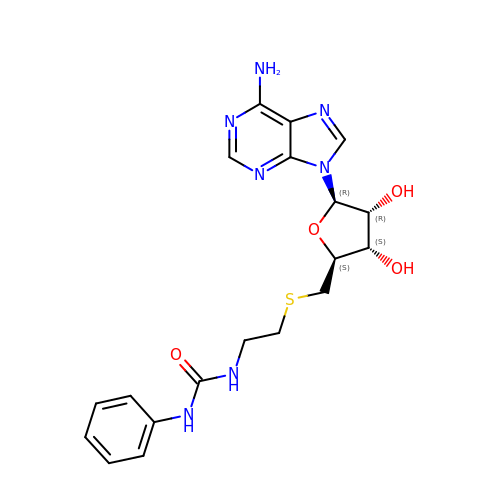5'-S-[2-(phenylcarbamamido)ethyl]-5'-thioadenosine | C19 H23 N7 O4 S | ZVEFVGBDFYZLDZ-SCFUHWHPSA-N>MQLGMIGLGRMGANIVRRLAKGGHDCVVYDHDPDAVKAMAGEDRTTGVASLRELSQRLSAPRVVWVMVPAGNI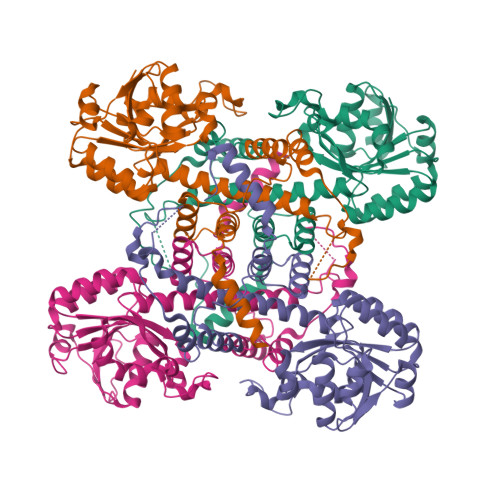TTAVIEELANTLEAGDIVIDGGNTYYRDDLRHEKLLFKKGIHLLDCGTSGGVWGRERGYCLMIGGDGDAFARAEPIFATVAPGVAAAPRTPGRDGEVAPSEQGYLHCGPCGSGHFVKMVHNGIEYGMMASLAEGLNILRNADVGTRVQHGDAETAPLPNPECYQYDFDIPEVAEVWRRGSVIGSWLLDLTAIALRESPDLAEFSGRVSDSGEGRWTAIAAIDEGVPAPVLTTALQSRFASRDLDDFANKALSAMRKQFGGHAEKPAN[4x]>[2x]MTGMSREEVESLIQEVLEVYPEKARKDRNKHLAVNDPAVTQSKKCIISNKKSQPGLMTIRGCAYAGSKGVVWGPIKDMIHISH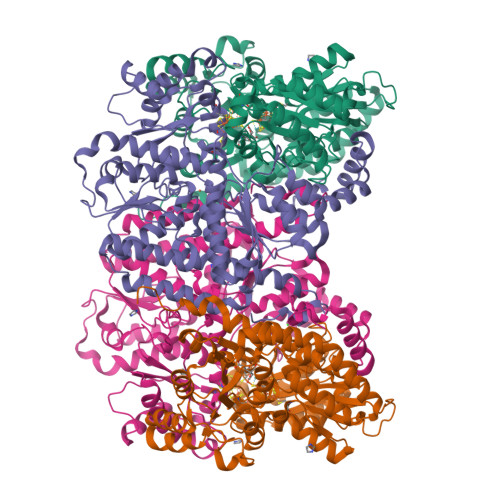GPVGCGQYSRAGRRNYYIGTTGVNAFVTMNFTSDFQEKDIVFGGDKKLAKLIDEVETLFPLNKGISVQSECPIGLIGDDIESVSKVKGAELSKTIVPVRCEGFRGVSQSLGHHIANDAVRDWVLGKRDEDTTFASTPYDVAIIGDYNIGGDAWSSRILLEEMGLRCVAQWSGDGSISEIELTPKVKLNLVHCYRSMNYISRHMEEKYGIPWMEYNFFGPTKTIESLRAIAAKFDESIQKKCEEVIAKYKPEWEAVVAKYRPRLEGKRVMLYIGGLRPRHVIGAYEDLGMEVVGTGYEFAHNDDYDRTMKEMGDSTLLYDDVTGYEFEEFVKRIKPDLIGSGIKEKFIFQKMGIPFRQMHSWDYSGPYHGFDGFAIFARDMDMTLNNPCWKKLQAPWEASEGAEKVAASA;>MSQQVDKIKASYPLFLDQDYKDMLAKKRDGFEEKYPQDKIDEVFQWTTTKEYQELNFQREALTVNPAKACQPLGAVLCALGFEKTMPYVHGSQGCVAYFRSYFNRHFREPVSCVSDSMTEDAAVFGGQQNMKDGLQNCKATYKPDMIAVSTTCMAEVIGDDLNAFINNSKKEGFIPDEFPVPFAHTPSFVGSHVTGWDNMFEGIARYFTLKSMDDKVVGSNKKINIVPGFETYLGNFRVIKRMLSEMGVGYSLLSDPEEVLDTPADGQFRMYAGGTTQEEMKDAPNALNTVLLQPWHLEKTKKFVEGTWKHEVPKLNIPMGLDWTDEFLMKVSEISGQPIPASLTKERGRLVDMMTDSHTWLHGKRFALWGDPDFVMGLVKFLLELGCEPVHILCHNGNKRWKKAVDAILAASPYGKNATVYIGKDLWHLRSLVFTDKPDFMIGNSYGKFIQRDTLHKGKEFEVPLIRIGFPIFDRHHLHRSTTLGYEGAMQILTTLVNSILERLDEETRGMQATDYNHDLVR[2x]>MWVDFIDQTKSLKVSVNNYFYYLDRIKKLFTYLNDLRKHILKKYVYTINHKRIAINYLYFSMVTGLSGAALATMIRLELAHPGSPFFKGDSLRYLQVVTAHGLIMVFFVVVPILFGGFANFLIPYHVGSKDVAYPRLNSIGFWIQPCGYILLAKIGFLRPQFWRYYDKTSFSFPFLEKMKYNQYKEYKNDYLFYLDFLKKEITDDHSFFWKARKVIKLPQYSVFSFVPLKLMMWKTMINYPESFWYAASRVVQSRRKKVFVTKCSARTLTTAGWTFITPFSSNIKYTAVGSQDILILSVVFAGISTTISFTNLLITRRTLAMPGLRHRRVLMPFVTISIFLTLRMLATITPVLGAAVIMMAFDRHWQTTFFEYAYGGDPILSQHLFWFFGHPEVYVLIIPTFGFINMIVPHNNTRRVASKHHMIWAIYVMAYMGYLVWGHHMYLVGLDHRSRTMYSTITIMISMPATIKVVNWTLSLVNGALKIDLPFLFSMSFLLLFLVAGFTGMWLSHVSLNVSMHDTFYVVAHFHIMLSGAAMTGIFSGIYYYFNALFGVKYSRMFGYMHLIYYSGGQWVAFVPLFYLGFSGMPRRIHDYPVVFMGWHSMSTTGHFITLVGIIFFFLMMFDSHIERRASTSTTLGLPRWYKRISYYIFKIRYLQHTKSKMNGIPGSTVRLMLINRHFVEYEVYEK[2x];>MWGNLWTEASYQLNFNIGFSSLRSDVLIHLAQWQYWWWFWFALIWSFYYFIILKVARFRVLKMRPKISTSYRPHGKWGDFLACIIPLIWCINILTNSNLILRLIEWQNESSLFTVRVRARQWYWIYKFELKNFTDILSTPKNIGNNRWQINTFGELQTADDYLHVLQLRSQNKWVKNYWNRSLQETGKTNKAHVISPQEQLRLSLINQYKSLNLSSSIKHNAPFINRDLYVFDDLFSYNLGDITTKKSLFNDKNSFLTSYSYLNNNSWNNNEFDLIDNLPFTTLFDNNDLFNNYKSFFQDSIFNSPKKQLSSDSKQLFKHIIYRSIKNNIIQDYTKLVKHEDFDEYSRWIKRSPGEVLPLRIIKYPLGLETIHNNIFENTNNEGNVELFRLRFNSNSSKMQHKLVQDTIYLTLKQKRYNRKKVVAPQIKYYKDDNGNKTDLVKYTGKPYLSNDKLLKQSIYDQTTQYKLIKKNKKRGELIPVTLARRILRTKKTLVLPAHVNITLITNSYDIVHSWFIPGLGIKLDCVPGRSTHHTFFIDNVGFYYGQCAEICGRYHHHMPIRVCALPFEHFLLWWNTFGLPKMLNTVSRKRFETHYELRKYSW[2x];>[2x]MLICNFLMYSNFSRIYWFDFNGTVNENLPLNYNVLKICRNEINKLEKLNENNLGTQKNPIKLNLSFEDKHYNTNNLVLDLNSYETFNSKNFISSIFDKTFESLNTVLMAPIYSFLEFKLKLSSTKINTNHYYVINGKLYITYNDSFKLFTTINDYFNDLNELSNTKLFFLYRSFNIYNIKLNSLVDFVFLKLILFIHLLYLKSTNYNRFDYRLKQTDWGFYINNNSNYIQNIFSGLKYIWRGLRFWIIGLLLGLSSIYYLMYVRLLPFNKIIFAWILVAMFLYWLLSGFVFFVKKYQYSKFTAAIQRFWKRTYIIFWVIEAGTFSVFFYLTLNASSEPVYMYDQIKIYKTHLFSWRWFLIKLLPSVSIILLGYYLQLTLKWNLFNKQNTIVLLITLLLLYILWLEFYQFYHILSFYGNINWAFDYDEYIWTLELDTRRTRLANNYIAICLFAKFWHFVFIFLFWVFFVLRINELGRIRYPLLVANVQNFIIIYIMSWAYMYPWLKFIFRKYLDVPYYWFYLNGRELGIRVFFTDLKLFFYGITNRLFDFNPSSIKFEKYPFYYWINSSQLTEFNQYRKFVIRDSIIYSLNNYII;>[2x]MKKQKRTQGKQNTKQIKQEKLSSKRKANNQKEGKKKVKQEDYKEIKQKGKRMLSKIVKASFSSKGFNLANAVNTVKSTLNAPIKHIKRNIEPTGSNYSRMTNTTEEAFDEVSHEWQALVTSNPFDLNVFNYLENTQTSNFGTVDNPLVVFTSETPFRYVGCTGQMNEDDYEGHELLFFLLREGSLQRCMGCGQVFKLVRLRNEYSPEMDYYLSNFHPYEMQEMGESDTTVLMSPYKYASHYEYTQFETPSNMVYSMVNPDEHDRLLVDPAYRMERTKALEEKYKVYTSSLREVEKQFEERYGRAGQINISKVTYSTLIDVEKAVLKMDRLFRKVAKFENRAFIDRANHSRREKRMLERAQQRWDSNYSFFTGSLTEEEQKYRDYYETELEAYPEDEGIEQQLDQQEVLLSGRYDPKLYDFQEGYTKNPEDDQTSLIEKKAFKFRYRLANETSETFQRRNNRMVERQIKRFQQPQYKHAFEQLQKNIAISSNSGNALHSEYGYLELLSNESVQLYKDYYESDAEEDFKVFENLSSKEKLVMIANFENNLLPKYDRSEVHLIPKRQWEPAFGVWENFLYDITEYASFIAPRGKEIAADYQIQSAIPLTKEELIEAGLYKETIEKKVEPKLEAKKQTKSE;>[2x]MIWKYLQRTNRGNIIQAGLQHRKFENLPFKQNFDNLTKAYDLRMWYISNSPHEAKNLEYVNELEALHNELNYQNSRQFLFRTVSFLLGWALFYQFYELPKTYDWQDTQEPKHQVPAYGDLEEGGDEGGDD;>[2x]MSSAVEKKDLPADYGKMPAGYNFLTRGKDWREYDKDFILRTDAVWEKFQLEHFFRNYMKCFFFDHGLKKYQMFEPEDMYTVVFEGWALDDLITFPGFTPTGRTNSYQIGLSPRQRTVVPTQTFYQMQDYYMLCGLRFERWFRCDLVYHDQRHTKFDQVKNQKNYKTYPCYREYYEAQYACQDDMFDFLMELAYARRAADNFESDFASHELTTLPTFYDTPKAAERKTYTY;>MGSVWFRNRYWWYRSLYDDYVAREAKLAFGIAAFIWLPHYYWGIHLNRAFEVNFSHRNYAHEWGPRRNRLAHSLEFEQFDMILENWQDLEDEYAQRGDGMLKK[2x];>[2x]MNRFFKVSSKYQYYKYLEQYDAAFLRKYQSETHWYLGRRGAWKNLVIKYAGDHISLEEEHNVKYKTHLSFVYLSYRLAWVLFAYVLIYNHFLLGDIGKTFNVGEWDHRLKPSAERDYPTRYESLYILDRTQKW;>[2x]MISKYRYLHCARKLVKQSVQAFGGGHHHHEYDWRDDPKVNKDIEEDIRDRGWHPETYDFPYTKKHDDWVFDVTMPSQNYQTDLTVNIHPENKKMHVMKQVMRQSYWDAEHDMAHEYDYESEDLDFQCESFKSQHFRKKGPISQYLILGLLPILYFGTEFFYNHYPDEDYWRVAHPPPLDYPDTDDTDDTETFKDYKSFTGRRMVDTGIVDPLWYDIREGKKVYYDWAGVNQPMEDI;>MSLSLFGVKNNWHKNGIWWFSKILNKTVGEERYDALRVQRRIWSMRFYYARQQCLYELFVDHPDLAQWTGTYPKVDSSHGFPFYSTYEMYRDFQENTLNSDGSFAQWITLVCGIYVIHVIYNYMIPYYWVSTPLKNDEFTRLRMKDYIASTVLEEVYGISYAEWGWLPHDFAYNRMRGLAGYMHPDDPRAMCTSTFHRKHKYIEHEVEKVGDYHHMTYPK[2x];>[2x]MNKSQDEVKEDYFSIKKKKYNSLDCVLSPIVTRKKQESINSFQAGLQEDQNSTAVPESPFIRNCSETLNRSQHKILDHYFEYDYSLKKKIEKIKISLQNKTGTDSSQSLVQKRLDDLRKKTLIYKQFNIQKNNNNINNTGQFFIEKDKQNNLNLSQPHQIIKSKQGHKRSFTNTLYCSSNDKKIFNISSQKQNIKTVKQSNNSSMYEEQIKNDQNKKQNFNKQAKSERKQAEFCDLFYESMQKDAERQFKSNSDKSKSITQILENNCENAIVLLNHLIQILTDSIPISKNSILLDEKLSQCVNLSNNSKISQLMLVIQKLQGKISYYYNDFLKCIRMMKICKNFCQLFGTLKFKISCYKYIGLGFQRLNKPKVALVYFVKMLRQSWFLKQEDQEINSYDFIGMSYFYLGSIDKAYQYHQMMIDGIKADEEVKKISNIMLKNRKYSNYPTLQNIRIIQETSDGQPLQKTIRKSKIINPQFQLTQQEWGENISSSEDEFELPQMQIAVKNAEEQTFQKKFLSTPWNDRFIQAQIHKLEIAQELNYNKFPIGLVFKNQSVLNFPNSSNQPQLVVGPYANKIYNQELSSTYSSRQRISHQTPNREFFNYHSQLQQVKEQTQLNQMKQQYNQIVDSIELANHLIVLKNLKKVKDLFQNLIPYLNEKYYNIKQQNTKSLKQQQNSFDAQNSNQSFLGLQNYSIQINGILNINNQTDEYVNNQSDRSYQQQSDKLKLLIKSKSRNHSKEINMTQNYFKSPSNESKQIKNLRVIVDNSNKKKAQQKLNQEFSMNFCESPKYDNSILSLFINKLSQESALRLEIRQIGSASRYQRKKQQKGKQRKEKYQKKQEENKLNIKQYKKERYNMALFFMANTAISVPSVLDTSPCMKQMLAYEDCVLDANVPQQEVIHPQWPTIWPRLLTDGKLLEFDKVPFHPENIYNYTYMRPLTKKNKQYLYECEEERFVFKACLRKVISLKKTDKHTSWDTAEVANLQLT;>MYLFMHLCMCFCMISSSQKKEKLNKGKNKQIKLNKKKEKQNKKIEIIKKEKERRSNPQMISKTQAFARLFQLSSKSFSTVKGGNLYTWGQYASGTGFETASAVPRKVDYFSGNVSKVAMGPYHTAVITNDGSLYTFGWGQNGALGNGAKEFQLSPSGNLYTWGQYASGTGFETASAVPRKVDYFSGNVSKVAMGPYHTAVITNDGSLYTFGWGQNGALGNGAKEFQLSPSPVSFFNDKKLKVKDVVVGESYTIAVTENGEVYSWGYGGEPSSKINLDFFRNAILPQRCGALGSGDNKNRLTPQQIANLKADGYKNISGGDNFATLVNQSGEVINWGTGLFGSLGNGSDYPLFTPEVNAYFKHLKEHEGLTVQSIKSAGHFSAALLSNGKLYTFGVNTQGQLGIRENLGHNTDQNARLPTPVVDRHFVGQKVVDFEVGENTLVFLTDKNEVFFSGLELAYQPIRWEIPTDKKIVKLAASKDTFAAVTETGKIYQFNEFVGVSTNEVGNDYNVADSKAFEGKVVDLGGSYGIRFAIVN[2x];>[2x]MLSKVTRRFLNYNQIYCFASQHGAEHHKLTASDEAYLNEVRQRYVTPDMEKWAYLDYKKHPSTTLSHYDHKSKDYVESERDDYNADVATNSHNKLIDDFKRNLQMQRKVHDILQKMDRPYLRGVPGVTKNISAGLQDYSAPVSKKSQSDPNDFYRDAYRNENRWIDQSVFTPKTSKMTHYDVEWPKELASRPVTKKFHHDKGYKYDVTTPYDQRYNYVADRLGHPEILGNPFERLMRLEGDIYHPNYLDQPFVKVPNANPNASLNFEEGEVLYENTRLLEWAKFWNYSVVVGYLWCAYFVPYNIFFKTHMPLEHAYDNLFFPYFQHTHFLWDNNALHIPTVGGVAIYATYIALSYINNIWKDYVVRAQFSKDKELLFVTRVSPFGTTEEEVYEVAHLEHLPPSVRSGVKDLSAQDADGLVDVTCMSSQRSLVFYKGDQYWNPKVYNDFINQTSNLWTRNYTGYNRLEVQNSVEQVKIGFSHSSQPKLEKK;>MTALFLHILWSISYIIINILYIFLSLLLSNNNEKIKQYNSNYFIKILLVLFYNKNLSFYKNLLSEDEISKIEFERLKNYPTLVLIHSNLNKLEKRNKIINSFINFKTKYRFYKFISTNFNLQTIIKNCNDKIIFSTLLYIVNLNYSFFYKTIKNTDLIVYLLANKFSILNDNIIVSKFNISKFNDYIKYINNTNSIDTYLENQIILGLNNNTNSNITKNINTKLLNSYSNLKNLVNITNNTFYLKKINDNYNTVINSEFLTYLKSNYKISFSASNIVKYLSDKSVNNSVILYLRKNKIFNKSRYSRNRQTYRTGAYWCLYVNIIAVVAFYFWFYKFTMNFGYLWWLLYSLILSFFFSRALKHRFYNPLNVMTEFKNGFMWFIIILINIFKPLLKLLENNYINLYNHLVIKYYQSFICNTLINKKKLEFNYILSSFKFIKELNNIIIISLNKLF[2x];>MFRRIISNGALLSTQTQRWQDLSKFACLRASLNKESEKAFQELAKKNNVSPQELVELSKIVSMNLDVLKQNINSEQFLLEKESTLKRYRQSSIGTRGHLQTVNEAVNTKYPTLAEGLGQVAGYKEAYQALREIFVHPSISVNNLRQGSYGQQFAVDFRTRADEYVKALLKDHSSNPQAVQTIQEIQHTLHQIIKNYEQNPASIYARILTVLQTRGVNTLPVSKTADQKAVATIQKTSTPSLTIDQLTVPVQERVQTQTVFDAELAFIKEANEMIQQNTGNLPWDGGKKKIFQGQANKYLETPYYLLAALSGLGLLYFLYSGDAKYKTLVLTPVVGIAAFVLLRRNQILNRVPTLTELFLHKDGKFVDAVVSVNGQLISKNDIPVSTLKLYRGDHTVKVNLNDFEDASAKKFLAQQSGQEGVINVHFSKLRNLAARNGQVLNLGDTEVVVPFENQANRIILKQIFKGVEVLPSS[2x];>MYEGRWKMVNQIKQDVQNDIELILRQMNERIHAMKKKKYNELKGKIKQKCIDLLIDYAKQKIGKKNKIKKEGNNIRHNKQKKLKNIQKKIFKIISTRMLQTTLSAFRPRGSNVTGKVALATLGALTGYGAFYHYNQYLNLSARWQQIQENIAKDQPFDVDGFDAKVYPWVRENNVNDWEYKLVKMRGYFKDQRFFVRRKRDGKEGFLVFAPFVTAVERVNHRLKQKDLLPVEYSVFVNLGWVPVENKKDVELGGEVCPPMDAPTDSTLFVNDTFTGFNPDPANPEDTEQVTLTEITGIVRRGEQQDILARRRNWNKEGIYNWVDLDYMGKIFRLFNLDAINTAYIERVVPSFEEGEEGLYPIPATKDTFERPLNTPERHSTFFNFYAATSALSFISMLLLRR[2x];>MISARAVHRFLRNPNLETGAAFRAGTRFDPFKNTLTVLKDPQNGRTLYLIGTTNSSTLLANRTKDLVQKEKPDAVFVQTNKEWWNLAKNIQDVKCQQELNRYNDLLSQAYTLSLDNTIRNLVFKAKFYSWLFVINWFKAFPDDFHPFIPGLEMKFAIEEANKQNIPVVLGGLEVDDVTLSALKVEPRLDPFSQLYYGYRALHNSFWRREHFDNYATLDVVGGEAYAESMDRFRTNWFVKYFEKLAPYQKKIIVDQKDLDLFYALYRDTPGKKIVAVVNQWHVPGIENHWKSATNTHEPLKAINPIGDMDINKYMESQLVNDTLRAFVSKVGKTEPATWKNYSTIYHKDNYEAERVRHVAFVDHKDPHMYHGLPQDYDDNIKPKHH[2x];>[2x]MRYLKIEKEKLVSCKKQEQEVQRIRRRKGNQKLNSIAKQQRVKRRDYQQNIKQNKEVKNPKKLIKQQIINKVKKRKKMFRGLTKFNKVFALNSFKNSLVAVPKANLNHVQNMLEENLKYDAQKYNDEVAVIQKTSRIYKPTYTIEFNREGEVLVYSADPIKNSVVYFKYPYVLYEAAIPLFIWAWIYNPLELSKNAVNSLLIYPNIAWIPRMWYWRSLQYKIQKMYLLRGGKVAKIETQSLAGDRFTSWVETYQFHPLTQDQKNFDNQDNAEFLEDEGQLKYELGVQLDNLQEMGTTSQDIVINFMKEGTVHHPELFEAIVKGYNIDTSDYVINTANNLRAREGNHNH;>[2x]MFFELEDIKRRHSLYWDIYNVQGWVRRPDSTLYNNVKRGVTAGVVASLVQENITALVENCKLLATKYEKPQNLRQAATFMKEVFKLENYRKAVWNRSQYALCIGTFDIGARLATFRWLNNGWQRVFAGFEFNFVRKIPTTMLAALFTAPFSVPFELARMAYYGDKTFPKELQRGYSSYLSALARIPFEEGPYFLFKNSFPLIIRNFFQTFTLFYTYDFLKDKASFAWRVGEQNEYACKMIIAGISTYLAAVFSYPWMVTREMVDFWPKVPGAPCTFNGNYRKAAVWIWYHEFSGNYFAGFFTKYFWKASPGMFLTLMLADKVGLFDQTTVDNFGGAGNNSWEDTFV;>[2x]MFLNRLVKETSKAKRLFSMAQNNFARAGPYNPNRYKDYYIPRTLPKNEEIVEFVQSQHSVPASPIRNQRHINPVRESGPLPSYDGTYTMEDIRAVFYNTTVGRDYCYCQMDPEEIMRRVPGITRKEAEFITKLGLSPQEQVDFAYIAYNIGLDIFYFTNQMFVARQVVTNSKGEKVEVLWNAQCYEDIAQLNVGFAPVLESVDYHWEIFLWADPPIKPNNDFDLNVPCTWFEYEQEWWMESCIQEDQFNLPEDERPYNTPRNPHCRKELWRSQDALQEEELMVNENWYPKNTQYNIYNQPDFIKPKSGSGAAADDIRI;>[2x]MANFVIPYLKPVADFWNSLCIDQHQDSLFQFKGQTGSLGTDWTSKYLRSEQDVYNHKYLQYHKRVHEAPELTDVISDNVYRLTLFAGVERVLSVRQAQAILKTQFAGATENISGAFQTVLNGGIFRRGYFRGALLNLLQFCGAPYQSLIWSRNSGITNQVIVSSIFEAFFYPLDTVKTLIYNDVQGKYKGAFHCASQVVQNAGWSRLYAGIFQKLIFNSALIFHLNQVWDGSSQQWASLALVAAAYPLLVLKTRFQVAGTPLALATSNEVLKVNRKTLYAGLVPYLIFNTLFAYEFAAWHSSTAQERVIGGLQNAMKQFSSPAAEQVWSS;>[2x]MNYSYKRYWEPSTAEVIGLSLSVNTISAALTYPIEFVKVRSQIRTEGVGIRSKNLYMGINPNKVFREIHATGNGLRGFYQGFESHLIGRLSYLFIRNLTYKIIYDRTKPVKAHNDLSHREKGVIAGFAGGLAAFLTSPADLVNTRTIAEGGKPKEWRWGYKGLMDGINKIAATEGGNAALFRGSYANVLRAVILNISLTGPFDYLNEKIWITFGDMTWNKYAALLWASFWGSVATLPFDNIRTRLYAQNADPTKNRLTYSGWADAAKKLIQHEGISGFYVGFYAFYIRTFLYAWTTVFITDKITSDWKRKAGLKEWQI;>MLQQVFGKSKGGEVTNSHLTPKVLNKAQEAEKLASQIQAQRFSNRLVAFSSQYPRAKLFFAGIGIGTLLYGANQSSKARENKVATETRKERMAKPTIQLTGADSQNPPFTEKNINDWLYKTVSITGRPIHGKGMMIPAKSYGLHGFEYLVPFVTKENEDGSVQEGLILNLGFIPREYAPIWARARVENVEEQTFTCVVTDGKHLSEQGGLFASNKPCENQWEYADLDQLAKHTGFVNQEQVRSCILEHVNTETPNDERDCRHIDICSDYKEDYPYKFTRSGVLQQPGQMYWDLNKSASYYSLLGLGCSVFSALLFLAK[2x];>[2x]MVYHLFERICNPDNFKLSGEAARVRTLIAAGFSKEEAEQVAWLQNHQVNGKILGLFTGGFALYCCNNYFHYFERYFPRLRYQPFTKFLAQAATVYFFFKIGDYYFTSRRYGSNDARMNGLMYSNTYYSTNKEALIQNFEPLNRKFTEEEVEQFLRNEGRSQEEKRNWIYNPHIHGSTEGEWKADIHEKFDSGKAPWEREHVKAKILETNKAKIDAGEEIQLKPFKTLNHLDKTGLLHRLHPFIWTNNWTLLG;>MSSFIQYEFLKIYQGNQKIKNYYKRKRLIFQQKKVLKKKQKEIQMSTNNLRLKPWFHWTDEERSHAIFSAYEKRILKSEDLPSFLRANRINNVSTWVFPLIALPLFNQSIFKLGFAQRILLTRPAIEWHCFKIATVAASWLAWLNFSPFYRKLENEKEYLLDTLESRIGINVLDLNDALPRWTTSQEYNRRTQQLYNQRNGFFAGLLYPQEESSRPLVDIASFPKNLHKEKLTK[2x];>MFGRLVLKQTRRTLFNPVLKNTFCIYQAYQNPLRHINTGHNPNNVYEDIVMLGDYPVQNRTHDKVISQTYVPAIANIAFTHLSKKYPQAGLKVDQLNTLKEKTWNDLGVNIEHEKQEILVELSEQIFVKESKLRWVHEQRQRLAHTTYVFSGLEFQNVKVGFFIDSYNFLLQELAHRSNLYQSKDIVGEKSFHEKHLEQQTAPYSGVKSLEEPVSQNKSFINSLMRAIHNH[2x];>[2x]MYVLFVCLIDSMNVEEGKQIKEMILPHNNRQLARQYFDSLPENDINRKYYEGLKYETPKTFFGRFLNQFNIDAKLDTLSKFYTYQKTIRATQAELQEDRKSYLTNSLLFTAVSWFSIYQFARKGAVLPVLREYGRYFGTHRLFRQYLHTLVLPLLYTEYALNQKYYTHMEHLWTVHVNRLNQKILEDPLYTFYPQELNVPKHNIIVPTIFRDTPQ;>[2x]MKKGTASEEELKKLYDPNTFYEHGDNPAFKQFMNIAVENLREGKLTDHRTYVVDTYKKWMYARNWDDFLQRDCKAITFPRAFALWIVGTLGMATASKWCRQILPVGSHGITKISQTQFFHQFGPLGTLGAVGFYGLTAYLYYKTTIFTVKKFYSHCILQEREWIFEQERQNPGYGEYFFKDVPLSAEEHFNDLARGEMAKKKFEKPNHEF;>MSALLKEILALTVKSEAALWKGAEQKVLSGLNNLAKTELVQITHHFGVNKQGSEALWSQLDKAAVGAFPELSVDETLQLIDGFGECPDSYTLSHDLNQRLLVSWEQLGKLNFQKLKETNPYFASDIVNQLDAAAAEFIKVRPAAESEAGGFLNSLGVSSSFNTTKNDIYVVQSASGKKLNNKEQREAYVLEKAQKYLKEDPQSKILDIIAQK[2x];>[2x]MFLGIFKDVIKLLNKKVVPVYFWFFLYCFLSTMDTNIFVSSCSFLKVEVFGKDENTTLVLLFYVFYSLFNFYLSRIKNKNNYLVRKHLYTTELLIELILFKYKLIILKFSSIKYILNFNVRKFILFNLFLINNYKAYKINTFFLYIYIYLNNLNIIWYPIFKAYSIFGYYKSTRLNFIDTKNENIKRIKY;>[2x]MKEKIFNELTRKMKRKEISAKIQREENKQILIRQRNNKKYIQSIQGIQQERKKGKLYLVEMATQNVEEMDTIQKMNYEATVNMGRQDLITREYTFYSDYEFIPIQEDRKQQMEDALNNLHKIIHPTVTQLKKKANVQEIQDRVFRKLQGWEGELNTCVFSAKNVRDSNFCADRFTNRINTEGVEFVKQILREY;>[2x]MSAILKRAAKYKRVSSILCEGEAHLRDPFTPPPVILKPPAPRKDKKPDDITDFPAQKLIPLPESIPYQEGKYRPASIPMVAGFFPYNCYLQQGKVYSWCSCGISQSGPWCDGLCNSVVTRCRPVVFNVSQSGYYKICNCKFSANAPFCNNTHRKMVRYHHQTHRGFYEIWGAALFVLGWVYMGFNYYT;>[2x]MAARDFEYNNQDVNQLNGAFISLVEDEKIGFWVGVGGFAYSQFIMRKFVKSTNIFASVTSLFAGAALANLYTHQSRASYARVAARANRNASLALNKLMEY;>MDNNYHFWGNGDRQDVSLSYEDYYSILDCLLDEKLSPQGLMKFKNLHEVSMYGVSYVPLYCFPVAYGISHMLTGKVRRGHSGYRNLFSLMSVVLPFTCWYAYTTPIPRRLYTEIICSNNADGAYVRNRIKQQKPGIWRKLSQQLYNKNFRFPELNQDLTATEFPLDYVAPHKF[2x];>[2x]MVFEFLFYNQQHKTRNGYFINHDNLMLASLEERKKLIFYFIANQVPEKLDPVDRVKFNEELSDNLSTKARLIGSLTGLIGLVGFPYISTRIYSRPVLNIGLSLLICPFLYYVGNQLTYSVWEPKFIANNNTVCELSKKYNFTVFDFAQAKKEAHLKALRTELVSDNLLYSPGI;>[2x]MNNTFKFLHQVISKLTLKAQVPNYGQYSHSLKRPINPKVVVFGNSSRAYELISSQFRNFNHVNGLELKGQEDNIQANKVAQSVLSINDGFQDGYYITDFPQNSKQAERLDLITDGVNLALYIKDPSDKVTVTRQQEAIDYYRKTGALVEFEVDPRGDLEEQVKQLSNQVLNGYKH;>MAIRNFVFKISNQIQNLAAKRSLAYLNQIDSQSVPSRATINMKDQVTQMQREIDNMANVIRAQIPDEDRAEFEILKKYYVTGQHDSLVDPQDVLLQLDRIQVLKNLKMIELNEEAYDPELVRLEKLKARVLLEEEGALLEYAHFISKRPYNKPYEKWGVSEEHVKQQILG[2x];>MGFETVVPAPPTRDDELRMIKATEEQFLQQPRYKLYMNEAHRIAKMNHGDRHNNIRAHFWSNFALGLLITGPIFIIPFGKAFRNLRSGVPYYFRPKYVFTQKNQYNQDRNWGAMKKQIPLWLGLSTAYAYWFTDFSINDDEWLEKGKVIYPHQTIKVL[2x];>MSCTTRRFIDEKEKLEYSRGYNQQELEASKLRKDFVKKYIVDFDTTLYKTQVERDWAYIAKREYRYEVQLKSIGYGGALANAVLLWRIYANKKMVFWPIPIVGALGYLYFQPVFFQKSNKRFFDMCNVGEEYYLGRERNKILRECNKILNVEDF[2x];>MGKDQLDFSHFDKAFENKYDIVAPEFGDLHQKRAEFIAKNQGTYRPVPLVPNNIKGLIPKTCRLPATRNWYRRTSSFERNGFFNIHTPVLNTKMIPWLLFIVLTWGWSSFQIGGYNYERFDDNGERRNTLYWKLSPVEFPQSKLWNRPS[2x];>MVFHYTNFVQETNAWWLRRVRPVYCTVLAYYGWWLYDRYYLFGKNATQDIRKDTTEVWEKRAALNKRNWGYNAHYKPELERSMKKVLYADPNYKFPIEWPERYMAETKTLEQVMDEEENWEYYK[2x];>[2x]MMQNLKKFMSKTIQVQPVSFNQIPKAFYNFPEYRTGGVQANPGITAKRIIKCIGERLRKYDPARWENVPITFKTHFRDENGYSDVATSIQIHDALEREFGIDIKDRLALVTDVETAFYIVMSHHDPL;>[2x]MEPFGTDERNWTHEEKDIITRFLKYDKHVNLKTAEMVYSAEVESAYFGKAGALAGGVISALFFNFPIVRNLPIIRRSVIGVLPFLYCYTWGKNTQEELRWLKTFAAYQRFVVYHGQHCKLWV;>[2x]MAQTAHQNRYQGGLCYAQCNELFSFWNPSIQQCWKGCDFGVGRVNDPEGRIEAQQMCKRWAAELYWTYKGELDTIKDLRVHADMYPTTPQNVYRACLAGVRRQKF;>[2x]MFRWLFLYWYNSTDTPSAIAKVNLWSYINLRLFKARLSSSIAYYILGLNNLELKKLKIFYKNTYFDYIYLKSIPCLFLIIFFTNLYLFL;>MSTRKIFDSEEQSFIRLVDKFYLGLSLTKLCAQSCNLLRNDISGSALTQKEKDCLSICYNNIEKTQSAFYAKVKTTMNLPAVEDDGEEGGDDE[2x];>[2x]MSSDPFKKVERDYHNERSVHKHFASYPLKFWWGLNKFETIQGIHSILGNAADLVVSTLSFIPGVQGRNNASYIENSIRVTRFRGFDDKTQ;>MEVKYRGPSDDKLECEFLENNLLSCLREKSVQDNVAKMTCRPEFLVWFFLECPTKAAVYHDPKGLRNIFIQDKIKQKGSDDGVLSKDD[2x];>[2x]MEDNYAADVQRQFNRTAFDSLYKICYNSLVQKNGSTIDFQKQIDCHQRLIQVFAKIAPIVVKVEQDAASSGGAAAGGEDEE;>MSDKRKIQHEGIIALINYSTLCAQKCDVLKGHDDKITDTEEQCLRVCAEKIRQTFEFTNDIYLKNPNLTKPN[2x];>MDPVLGDVIATRIYKACFKHVYGKNMKAYSEKDEAKFDQCLTSYVESYKSVTNHFITYLGQLPKKGLSLDGS[2x];>[2x]MEQNTTQVFSDLAYKVCFKVINDKN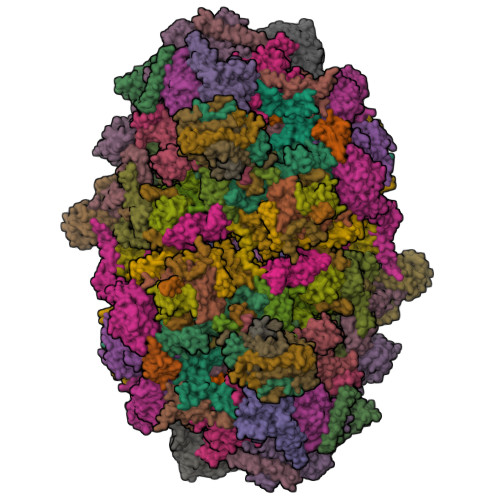KPFVLHDEQRLANCLTRYVEAFNVTSEYFFRERAGETKVTEKQ;>MDTEVSNHNYTQAVAYLNRATSSCVKKCDSLNNNGSLSSKQESCLKTCAENHAIATKIHAEYIRKLAESKYL[2x]>[2x]MGFKVKLEKRRNAINTCLCIGLDPDEKDIENF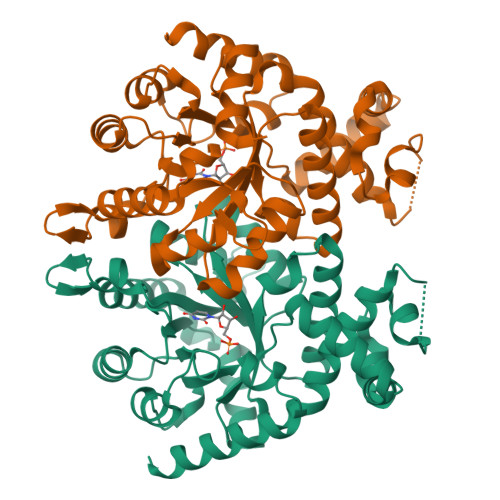MKNEKENNYNNIKKNLKEKYINNVSIKKDILLKAPDNIIREEKSEEFFYFFNHFCFYIINETNKYALTFKMNFAFYIPYGSVGIDVLKNVFDYLYELNIPTILDMKINDIGNTVKNYRKFIFEYLKSDSCTVNIYMGTNMLKDICYDEEKNKYYSAFVLVKTTNPDSAIFQKNLSLDNKQAYVIMAQEALNMSSYLNLEQNNEFIGFVVGANSYDEMNYIRTYFPNCYILSPGIGAQNGDLHKTLTNGYHKSYEKILINIGRAITKNPYPQKAAQMYYDQINAILKQNMES[1-(1-BENZYL-3-HYDROXY-2-OXO-PROPYLCARBAMOYL)-2-PHENYL-ETHYL]-CARBAMIC ACID BENZYL ESTER | C27 H28 N2 O5 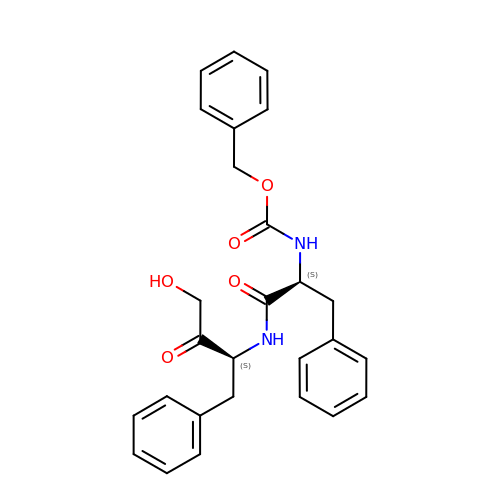| OACUXIVGLLCILS-ZEQRLZLVSA-N>MAHHHHHHSAALEVLFQGPGMASGSNVEEYELDVEALVVILRDRNIPRNPLHGEVIGLRLTEGWWGQIERFQMVRLILQNDDNEPLQRPRYEVIQRAVNPHTMFMISGPLAELQLAFQDLDLPEGPLRFGPLANGHYVQGDPYSSSYRPVTMAETAQMTRDELEDVLNTQSEIEIQMINLLELYEVETRALRR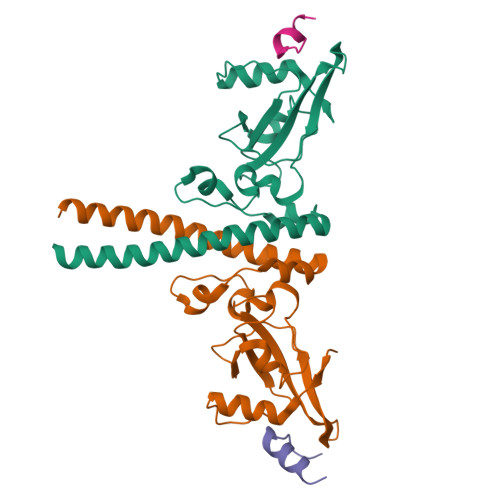QLAERS[4x];>[4x]MAPPMTLQQWIIWKKMNKAH> GPLGSEPRSLTAEEVKRLEEQEEDTFRELRIFLRNVTHRLAIDKRFRVFTKPVDPDEVPDYVTVIKQPMDLSSVISKIDLHKYLTVKDYLRDIDLICSNALEYNPDRDPGDRLIRHRACALRDTAYAIIKEELDEDFEQ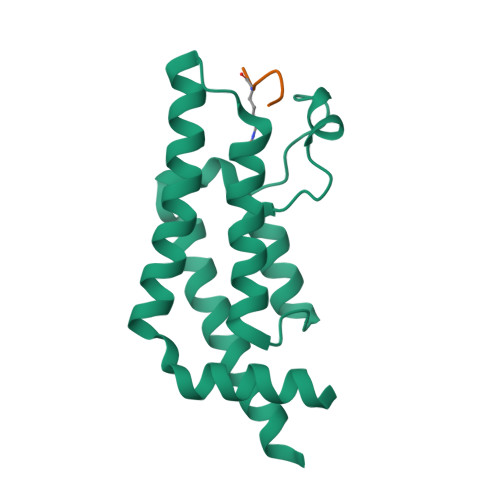LAEEIQESRKKRG;> CGRGKGGKGLGKGGA We show that the orthologue identified in A. hydrophila (AhlABC) is a haemolytic tripartite α-PFT, requiring all three components for maximal lysis, and we present the structures of the soluble forms of monomeric AhlB and tetrameric AhlC and the decameric pore form of AhlB. AhlC provides the initial single leaflet insertion, assembly with AhlB then producing an oligomeric hydrophobic pore, and finally recruitment of AhlA produces a hydrophilic fully active AhlABC pore. Structural and sequence analysis suggests this method of pore assembly may well occur throughout the tripartite α-PFT family.

Based on the length of the hydrophobic head of AhlC, its delineating charged residues and the observation that it is not lytic in isolation, we suggest that AhlC inserts into a single leaflet of the bilayer. We thus constructed a triple leucine to threonine mutation (α3 L156T, and α4 L160T, L161T) of AhlC to reduce the hydrophobicity of the head. Haemolytic assays using the triple mutant of AhlC resulted in an almost 80% reduction in activity of the AhlABC complex. We also determined the structure of this triple mutant of AhlC, which showed it adopts the same tetrameric structure as that observed for the wild-type AhlC (rmsd 0.6 Å) . In addition, the triple Leu–Thr head mutant of AhlC designed to decrease its hydrophobicity, reduces lytic activity by 80%, emphasising the head’s critical role. Taken together, these results show that monomeric AhlC is required for lysis, and that disassembly of the tetramer of AhlC and the hydrophobic nature of the head of AhlC are both vital for pore formation.

>MSNGILSQSIANMQQAEATIQSFSGLPQNAVNIQQNVGEVVAALLPQVQTMQQQVLAFAARLELQLTQQLANTGPFNPEALKAFVDLVQQEIAPIQTLTAQTLTASQSANDRITQDNIALQRIGVELQATIAGLQSNLDGARQELDSLNKKKLYLTGLGTTGLPGLIALAVTLTQTQNKVSSLEGQVNQIEGQIQRQQGFLGQTTAFSQQFGSLIDRVSKVGNTISLLGGDIANVARDAGQGDPELARLFFTAALTEVRTLQVDASHHHHHH[2x]> MKESYYSIGEVSKLANVSIKALRYYDKIDLFKPAYVDPDTSYRYYTDSQLIHLDLIKSLKYIGTPLEEM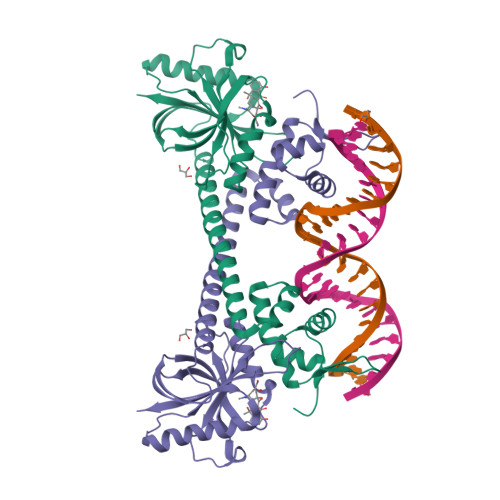KKAQDLEMEELFAFYTEQERQIREKLDFLSALEQTISLVKKRMKRQMEYPALGEVFVLDEEEIRIIQTEAEGLGPENVLNASYSKLKKFIESADGFTNNSYGATFSFQPYTSIDEMTYRHIFTPVLTNKQISSITPDMEITTIPKGRYACIAYNFSPEHYFLNLQKLIKYIADRQLTVVSDVYELIIPIHYSPKKQEEYRVEMKIRILD> SNAMYKYITILGAAGQIAQXLTATLLTYTD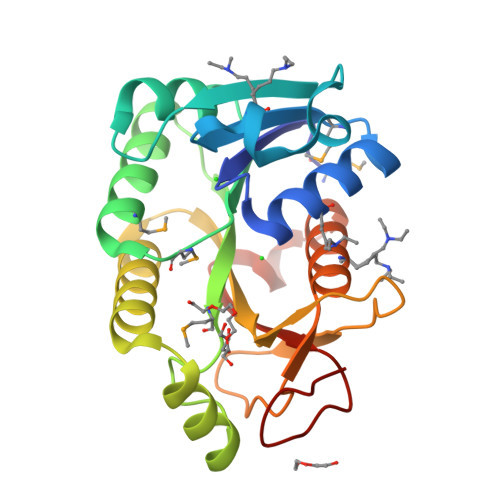MHITLYGRQLXTRIPPEIIDHERVTVIEGSFQNPGKLEQAVTNAEVVFVGAMESGSDMASIVKALSRKNIRRVIGVSMAGLSGEFPVALEKWTFDNLPISYVQGERQARNVLRESNLNYTILRLTWLYNDPEKTDYELIPEGAQFNDAQVSREAVVXAIFDILHAADETPFHRTSIGVGEPGTHYDKPSFH>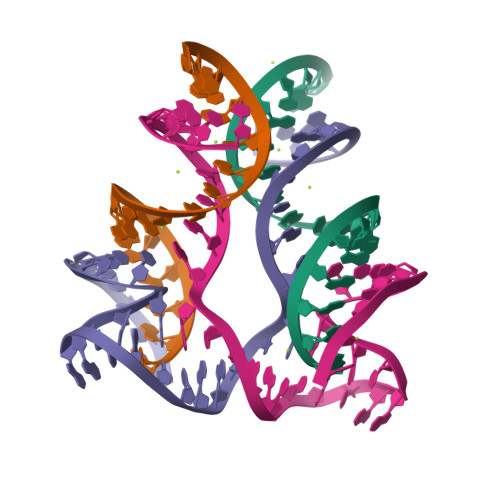[2x]AGGAGAGAGAUGGGUGCGAG;>CTCGCACCCAGGCTAGCTACAACGACTCTCTCCT[2x]5-(2-CHLORO-4-NITROPHENYL)-2-FUROIC ACID | C11 H6 Cl N O5 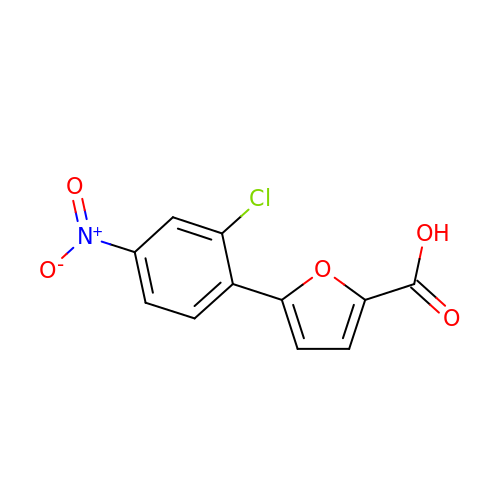| HDIHNBCCQWMVBW-UHFFFAOYSA-N>GKISTDKYIFLTPRAYIIVHLLKVGKAKASEIS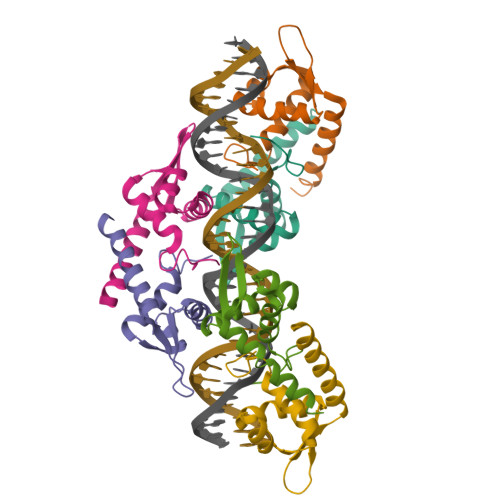ENTQIPYQTVIQNIRWLLAEGYVVKEQKGEEIYYKLTDKGKQLATAELEKIRKLVEVVQ[6x]>AEKPKLHYFNARGRMESTRWLLAAAGVEFEEKFIKSAEDLDKLRNDGYLMFQQVPMVEIDGMKLVQERAILNYIASKYNLYGKDIKERALIDMYIEGIADLGEMILLLPVCPPEEKDAKLALIKEKIKNRYFPAFEKVLKSHGQDYLVGNKLSRADIHLVE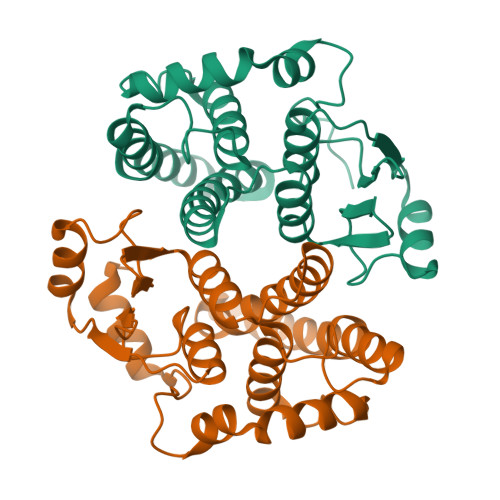LLYYVEELDSSLISSFPLLKALKTRISNLPTVKKFLQPGSPRKPPMDEKSLEEARKIFRF[2x]>MLAKVLKKRGAVLRGDFVLSSGRRSSVYIDMRRLLGDESSYSVALDLLLEVGGQDLARSSAVIGVATGGLPWAAMLALRLSKPLGYVRPERKGHGTLSQVEGDPPKGRVVVVDDVATTGTSIAKSIEVLRSNGYTVGTAL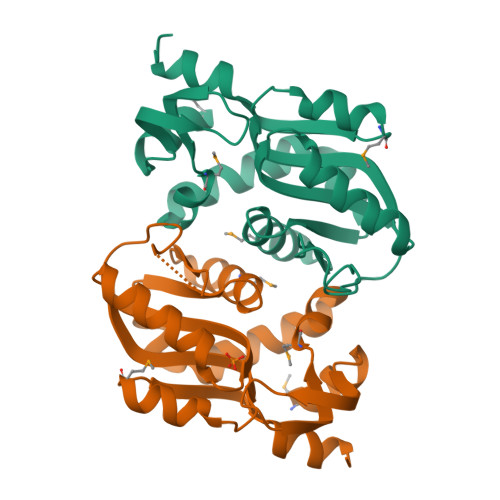VLVDRGEGAGELLARMGVRLVSVATLKTILEKLGWGGE[4x]>MTIQDIQSLAEAHGLLLTDKMNFNEMGIDFKVVFALDTKG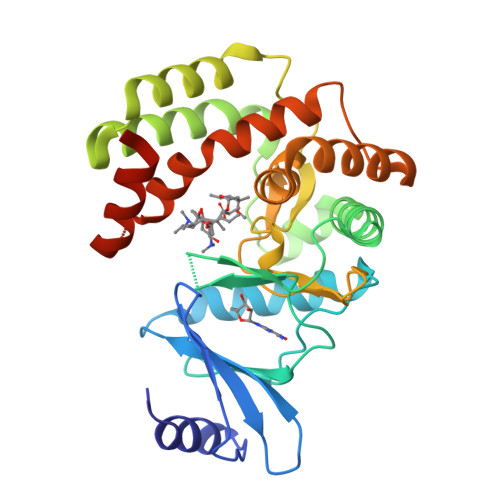QQWLLRIPRRDGMREQIKKEKRILELVKKHLSVEVPDWRISSTELVAYPILKDNPVLNLDAETYEIIWNMDKDSPKYITSLAKTLFEIHSIPEKEVRENDLKIMKPSDLRPEIANNLQLVKSEIGISEQLETRYRKWLDNDVLWADFTQFIHGDLYAGHVLASKDGAVSGVIDWSTAHIDDPAIDFAGHVTLFGEESLKTLIIEYEKLGGKVWNKLYEQTLERAAASPLMYGLFALETQNESLIVGAKAQLGVILEHHHHHH[2x]>GHMGTNRPLVFVDLDDTLFQTSRKMVEGTPRTTATLDVHGQPNGYMNPIQHSFISWLLASADVVPVTARDVEAYSRVKLPFTEGAICSHGGVMLHSDGSLDQDWHGQMAKSLWAFQDRLPALSEATLRIGKDMGYSLRGWVVEEEGLRHY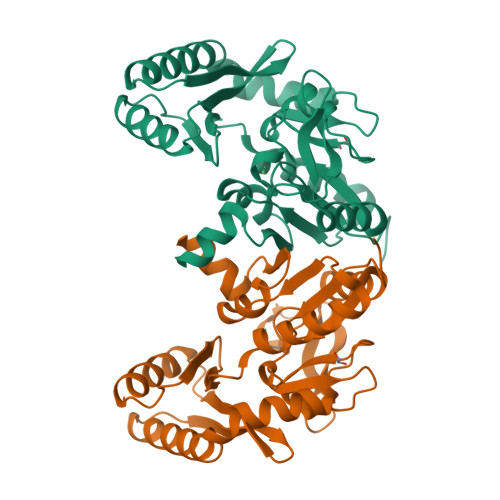VVTKQNESDDAVLSKVLAEVQARGMLEGMHIHANGNNLAFLPKGLAKRLAVQEWLRRDAKINGDRPVLGFGDSITDLGFMGLCHMWATPARSQLAKAVEEMIIE[2x]>[4x]HMEGPAGYLRRASVAQLTQELGTAFFQQQQLPAAMADTFLEHLCL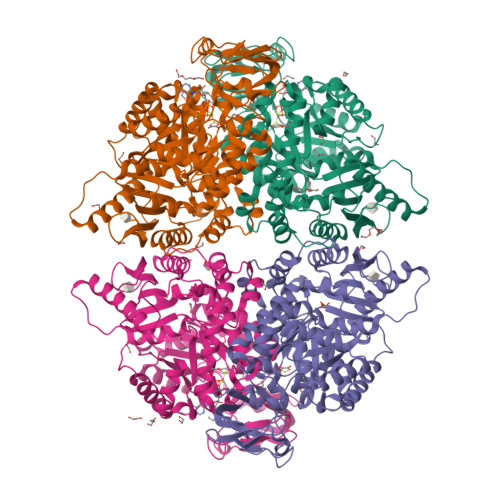LDIDSQPVAARSTSIIATIGPASRSVDRLKEMIKAGMNIARLNFSHGSHEYHAESIANIREATESFATSPLSYRPVAIALDTKGPEIRTGVLQGGPESEVEIVKGSQVLVTVDPKFQTRGDAKTVWVDYHNITRVVAVGGRIYIDDGLISLVVQKIGPEGLVTEVEHGGILGSRKGVNLPNTEVDLPGLSEQDLLDLRFGVQHNVDIIFASFVRKASDVLAVRDALGPEGQNIKIISKIENHEGVKKFDEILEVSDGIMVARGDLGIEIPAEKVFLAQKMMIGRCNLAGKPVVCATQMLESMITKARPTRAETSDVANAVLDGADCIMLSGETAKGSFPVEAVMMQHAIAREAEAAVYHRQLFEELRRAAPLSRDPTEVTAIGAVEASFKCCAAAIIVLTKTGRSAQLLSQYRPRAAVIAVTRSAQAARQVHLSRGVFPLLYREPPEAIWADDVDRRVQFGIESGKLRGFLRVGDLVIVVTGWRPGSGYTNIMRVLSVSHHHHHH>[4x]AEAGITGTWYNQLGSTFIVTAGADGALTGTYESAVGNAESRYVLTGRYDSAPATDGSGTALGWTVAWKNNYRNAHSATTWSGQYVGGAEARINTQFLL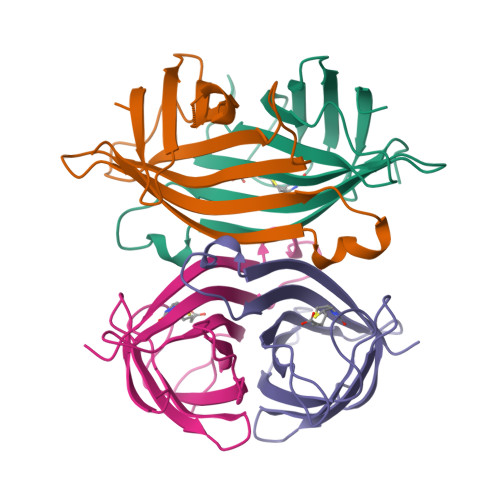TSGTTEANAWKSTLVGHDTFTKVKPSAAS>[2x]MELRHTPARDLDKFIEDHLLPNTCFRTQVKEAIDIVCRFLKERCFQGTADPVRVSKVVKGGSSGKGTTLRGRSDADLVVFLTKLTSFEDQLRRRGEFIQEIRRQLEACQREQKFKV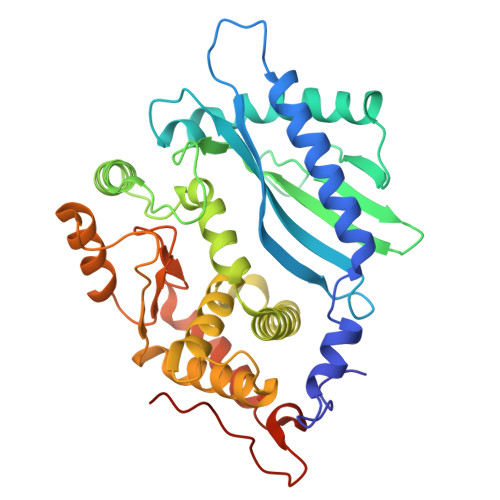TFEVQSPRRENPRALSFVLSSPQLQQEVEFDVLPAFDALGQWTPGYKPNPEIYVQLIKECKSRGKEGEFSTCFTELQRDFLRNRPTKLKSLIRLVKHWYQTCKKTHGNKLPPQYALELLTVYAWEQGSRKTDFSTAQGFQTVLELVLKHQKLCIFWEAYYDFTNPVVGRCMLQQLKKPRPVILDPADPTGNVGGGDTHSWQRLAQEARVWLGYPCCKNLDGSLVGAWTMLQKIGSHHHHHH> MDLKPDNYFSGQQLTLARAIENGEVDEVIKLASGTDLNKPGKEDMTLLFWAVMNSINNQKTPERLNVITMLIKAGADPLQPRPQGKNSPAEFVLMADNADWIKAMLNAGLSPNAVDKTFGKPIIFQTLEAKNTKTLQAMLDKGADINITDSLGNTLLIDALDFHSYD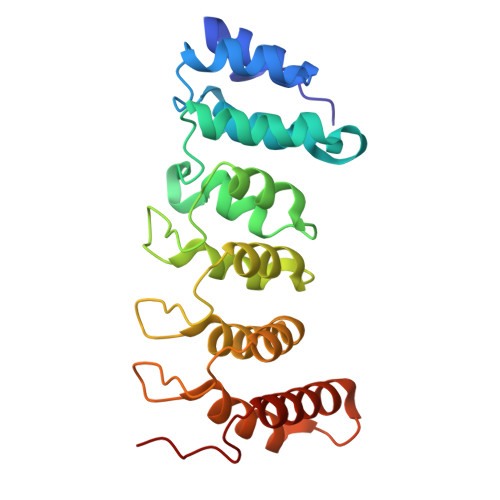HVLLLLERGADPEIKADNGWTMGNQLQRFLDRAKVGSDEYKKLNEIKDVLIQHGGKWPPTPVK>[2x]AAESGELIGACEFMKDRLYFATLRNRPKSTINIHYF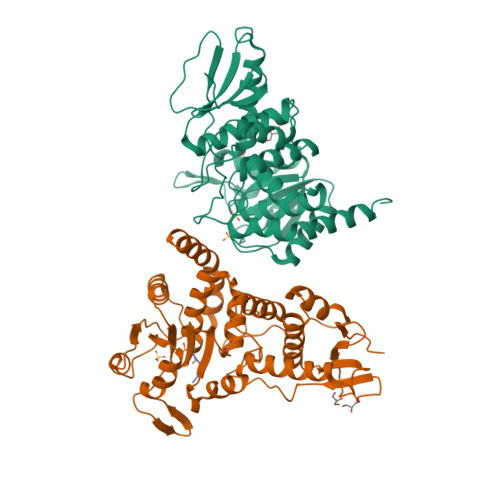SIDEELVYENFYADFGPLNLAMVYRYCCKLNKKLKSYSLSRKKIVHYTSFDQRKRANAAFLIGAYAVIYLKKTPEEAYRALLSGSNPPYLPFRDASFGNCTYNLTVLDCLQGIRKGLQHGFFDFETFDAEEYEHYERVENGDFNWIVPGKFLAFSGPHPKSKIENGYPLHAPEAYFPYFKKNNVTTIVRLNKKIYEAKRFTDAGFEHYDLFFIDGSTPSDNIVRRFLNICENTEGAIAVHSKAGLGRTGTLIACYVMKHYRFTHAEIIAWIRICRPGSIIGPQQHFLKEKQASLWVQGDIFRSKLKNR;> ASPRRR> MRWGYTSVQGFRDEMEDDIVIRSDAVDSFSYAAVFDGHAGSSSVKFLREELYKECVGALQAGSLLNGGDFAAIKEALIKAFESVDRNLLKWLEANGDEEDESGSTATVMIIRNDVSFIAHIGESCAVLSRSGQIEELTDYHRPYGSSRAAIQEVKRVKEAGGWIVNGRICGDIAVSRAFGDIRFKTKKNDMLKKGVDEGRWSEKFVSRIEFKGDMVVATPDIFQVPLTSDVEFIILASDGLWDYMKSSDVVSY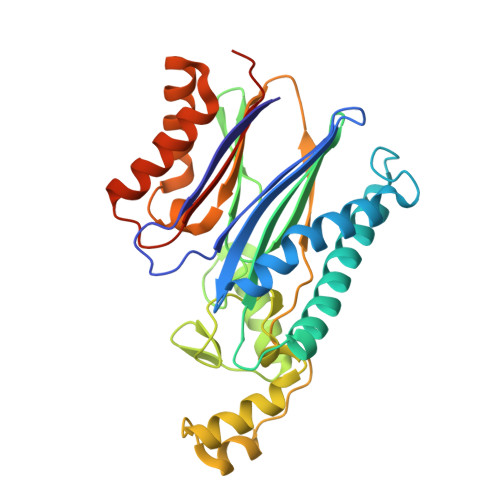VRDQLRKHGNVQLACESLAQVALDRRSQDNISIIIADLGRTLEHHHHHH> MSSNSLALKGRSDAYTQVDNFLHAYARGGDELVNGHPSYTVDQAAEQILREQASWQKAPGDSVLTLSYSFLTKPNDFFNTPWKYVSDIYSLGKFSAFSA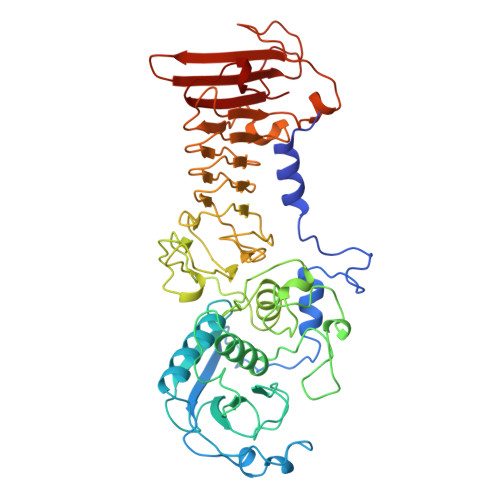QQQAQAKLSLQSWSDVTNIHFVDAGQGDQGDLTFGNFSSSVGGAAFAFLPDVPDALKGQSWYLINSSYSANVNPANGNYGRQTLTHEIGHTLGLSHPGDYNAGEGDPTYADATYAEDTRAYSVMSYWEEQNTGQDFKGAYSSAPLLDDIAAIQKLYGANLTTRTGDTVYGFNSNTERDFYSATSSSSKLVFSVWDAGGNDTLDFSGFSQNQKINLNEKALSDVGGLKGNVSIAAGVTVENAIGGSGSDLLIGNDVANVLKGGAGNDILYGGLGADQLWGGAGADTFVYGDIAESSAAAPDTLRDFVSGQDKIDLSGLDAFVNGGLVLQYVDAFAGKAGQAILSYDAASKAGSLAIDFSGDAHADFAINLIGQATQADIVV> MGRFIFVSFGL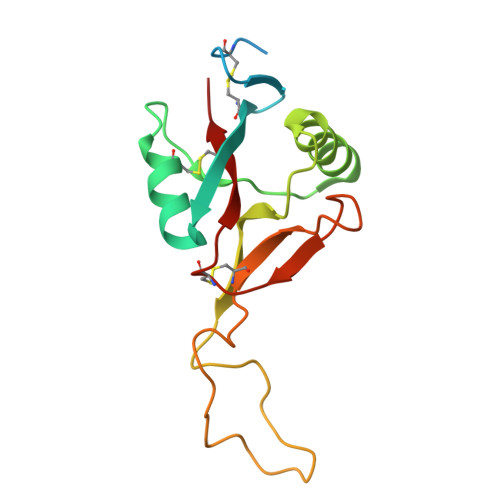LVVFLSLSGTGADVDCLPGWSAYDQSCYRVFKLLKTWDDAEKFCTERPKGGHLVSIESAGERDFVAQLVSENKQTDNVWLGLKIQSKGQQCSTEWTDGSSVSYENFSEYQSKKCFVLEKNTGFRTWLNLNCGSEYAFVCKSPP> ADTIVAVELDSYPNTDIGDPSYPHIGIDIKSIRSKSTARWNMQTGKVGTAHISYNSVAKRLTAVVSYSGSSSTTVSYDVDLTNVLPEWVRVGLSATTGLYKETNTILS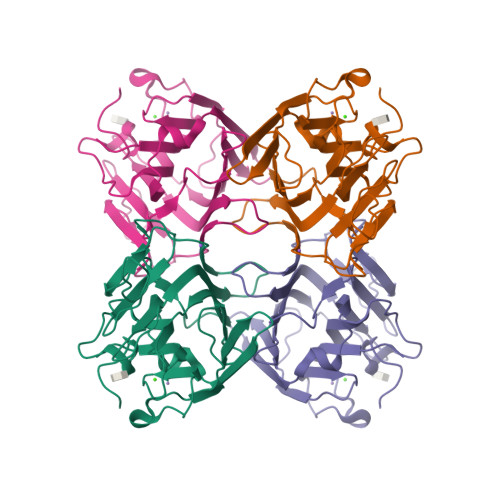WSFTSKLKTNSIADANALHFSFNQFTQNPKDLILQGDATTDSDGNLELTKVSSSGSPQGSSVGRALFYAPVHIWESSAVVASFDATFTFLIKSPDSEPADGITFFIANTDTSIPSGSSGRLLGLFPDAN Apicoplast replication, however, is carried out by a single DNA polymerase called apPol. Apicoplast DNA undergoes reactive oxygen species-mediated oxidative damage, and since apPol is the only polymerase in the apicoplast, this enzyme is anticipated to perform both replicative and lesion bypass DNA synthesis. ApPol belongs to the A-family of DNA polymerases but is only distantly related to the well-studied A-family polymerases, including bacterial DNA polymerase I (Pol I), T7 DNA polymerase, and mitochondrial DNA polymerase gamma. We have used electron cryomicroscopy (cryoEM) to solve a series of structures of apPol in complex with an undamaged primer/template DNA and the correct incoming dNTP.

The apPol density was well-resolved, and we could trace the entire polypeptide backbone and identify densities for several amino acid residues. Overall, the apPol structure was similar to the previously reported structure of the apo enzyme. The DNA density was fragmented and there was no clear density for the incoming nucleotide. We further classified the particles contributing to the consensus map and could resolve them into four structures (global resolution ranging from 3.8 Å to 4.1 Å) corresponding to apPol–DNA, apPol–dGTP, and two conformational states of apPol–DNA–dGTP complexes.

> MGSSHHHHHHSQDPENLYFQGDEITKKYIKDNIINVDDNIIKKKDIFKLKNENNEITECAFEYFESKKKFDDDIESRFFIINDNNYNENINLIYKDIKYCGLNIQTTGLEVFDENIRLIQIAVENYPVIIYDMFNINKKDILDGLRKVLENKNIIKIIQNGKFDAKFLLHNNFKIENIFDTYIASKLLDKNKNMYGFKLNNIVEKYLNVILDKQQQNSVWNNSLLNNNQLFYAARDSSCLLKLYKKLKEEIKKENLHIVNDIENKCILPICDMELNGIKVDLENLQKSTNEILNELNIEKDNLKKKLKDENINVNSQQQVLKALQKNNVRDISNKLIENTSDSNLKNFLNHEEIISLRNYRRLYKLYSAFYLKLPLHINTKTNKIHTTFNQLKTFSGRFSSEKPNLQQIPRQKNIREIFIPNDNNIFIIADFKQIELKIAAEITNDEIMLKAYNNNIDLHTLTASIITKKNIPDINKEDRHIAKAINFGLIYGMNYVNLKNYANTYYGLNMSLDQCLYFYNSFFEHYKGIYKWHNQVKQKRALQYSTLSNRKVIFPYFSFTKALNYPVQGTCADILKLALVDLYDNLKDINGKIILCVHDEIIIEVNKKFQEEALKILVQSMENSASYFLKKVKCEVSVKIAENWGSKD> MKSNEHDDCQVT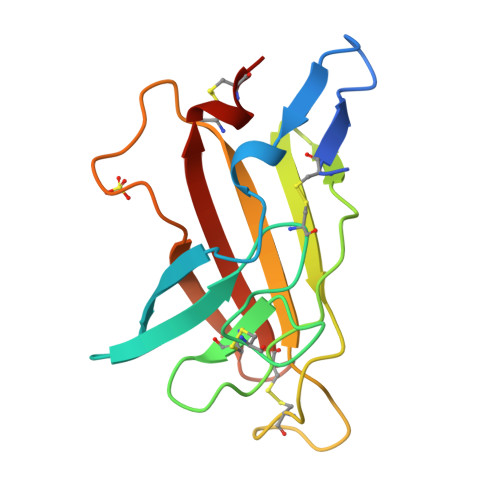NPSTGHLFDLSSLSGRAGFTAAYSEKGLVYMSICGENENCPPGVGACFGQTRISVGKANKRLRYVDQVLQLVYKDGSPCPSKSGLSYKSVISFVCRPEAGPTNRPMLISLDKQTCTLFFSWHTPLACEQAT>GRGYEIPARLRTLHNLVIQYASQGRYEVAVPLCKQALEDLEKTSGHDHPDVATMLNILALVYRDQNKYKDAAHLLNDALAIREKTLGKDHPAVAATLNNLAVLYGKRGKYKEAEPLCKRALEIREKVLGKFHPDVAKQLSNLALLCQNQGKAEEVEYYYRRALEIYATRLGPDDPNVAKTKNNLASCYLKQGKYQDAETLYKEILTRAHEKEFGSVNGENKPIWMHAEEREESKDKRRDSAPYGEYGSWYKACKVDSPTVNTTLRSL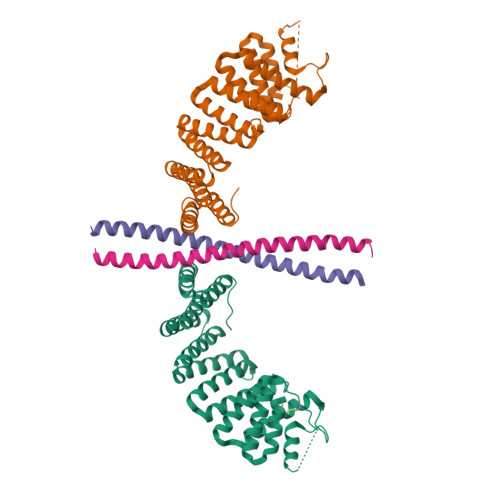GALYRRQGKLEAAHTLEDCASRSR[2x];>GPGGRMGKEVGNLLLENSQLLETKNALNVVKNDLIAKVDQLSGEQEVLKGELEAAKQAKVKLENRIKELEEELKR[2x]> IDITGDWTVAVYCAASPTHAE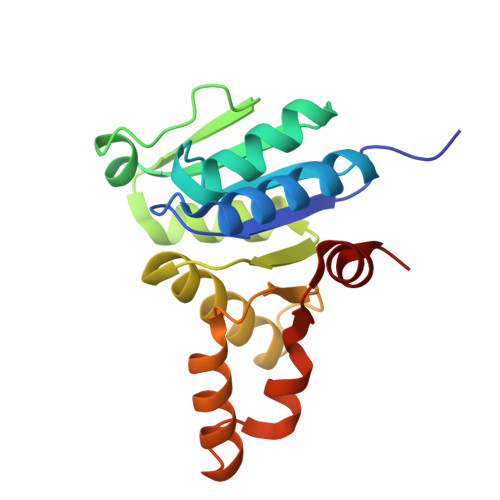LLELAAEVGAAIAGRGWTLVWGGGHVSAMGAVASAARACGGWTVGVIPKMLVYRELADHDADELIVTDTMWERKQIMEDRSDAFIVLPGGVGTLDELFDAWTDGYLGTHDKPIVMVDPWGHFDGLRAWLNGLLDTGYVSPTAMERLVVVDNVKDALRACAPS>[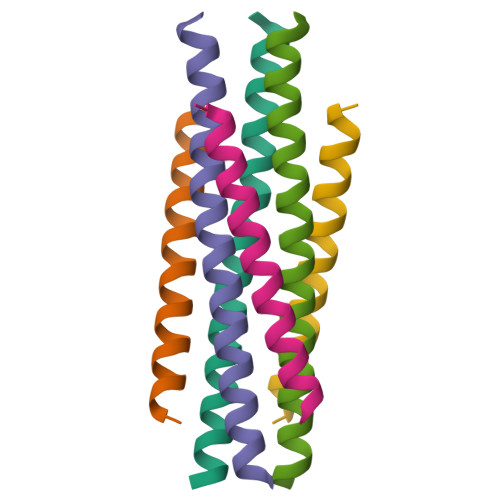2x]XQARSDIEKLKEAIRDTNKAVQSVQSSIGNLIVAIKSVQDYVNKEIVPSIARX;>[2x]XVALDPXDISIVLNKIKSQLEESKEWIRRSNKILDSIX>RGSHMEVRNMVDYELLKKVVEAPGVSGYEFLGIRDVVIEEIKDYVDEVKVDKLGNVIAHKKGEGPKVMIAAHMDQIGLMVTHIEKNGFLRVAPIGGVDPKTLIAQRFKVWIDKGKFIYGVGASVPPHIQKPEDRKKAPDWDQIFIDIGAESKEEAEDMGVKIGTVITWDGRLERLGKHRFVS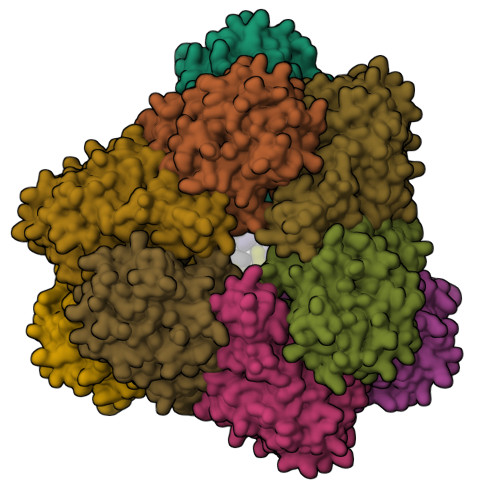IAFDDRIAVYTILEVAKQLKDAKADVYFVATVQEEVGLRGARTSAFGIEPDYGFAIDVTIAADIPGTPEHKQVTHLGKGTAIKIMDRSVICHPTIVRWLEELAKKHEIPYQLEILLGGGTDAGAIHLTKAGVPTGALSVPARYIHSNTEVVDERDVDATVELMTKALENIHELKI[4x]>NDELIKLEKEPGQWVMQNKNYANTRYSELNQINTKNVSRLRLAWSFSTGALRGHEGGPLVVGTTMYVHSAYPNHVYALDLTQKPYAIKWQYTPVQNSQAVAVACCDVVNRGLAYANGKIFMTTLDGQIIALDANTGKELWKMKHADVTKGETITGAPLVVKDKVLVGVSGGEFGVRGRVGAYDINTGNRVWLAYSQGPDEEVLLDSDFNKEFPQHGGPGDGTKTWPGEQWKLGGGTTWGWYSYDPALDLFYYGTSNPGTWNAEQRKGGDNKWSCTIFARRPDTGKARWAYQMTPWDSWDYDGVNEMILPDLTVKGKKTPCLVHFDRNGFGYVLDRRTGQLIEAQPFVYVNWAKEISKENDRPVEIPEKRTKQGVDTKGICPNSMGGKDQQPAAFSPQ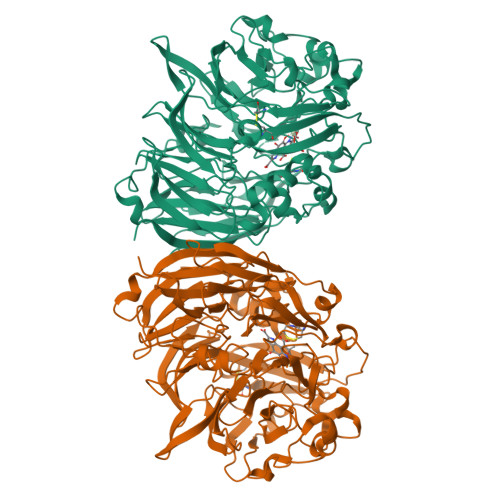TGLFYVPTNNMCMNYEGVEATYTAGAPYVGANVLMYSGHEGKDDYYGAFICYDALKGKRVWEIHEHFPVWSGPVVTAGGLAFYGTMDGWFKAVDIKTGKVLWQQKLGSGIIGNPITFLGPDKKQYVAVYSGVGGWFGIAVAQNLPPDDPYAGLGAVGVAYQAGLPKATTVGGELYVFALE[2x]> GAMVEATAQETDRPRFSFSIAAREGKARTGTIEMKRGVIRTPAFMPVGTAATVKALKPETVRATGADIILGNTYHLMLRPGAERIAKLGGLHSFMGWDRPILTDSGGYQVMSLSSLTKQSEEGVTFKSHLDGSRHMLSPERSIEIQHLLGSDIVMAFDECTPYPATPSRAASSMERSMRWAKRSRDAFDSRKEQAENAALFGIQQGSVFENLRQQSADALAEIGFDGYAVGGLAVGEGQDEMFRVLDFSVPMLPDDKPHYLMGVGKPDDIVGAVERGIDMFDCVLPTRSGRNGQAFTWDGPINIRNARFSE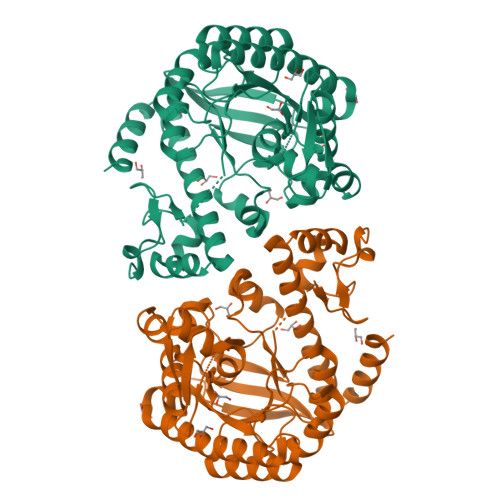DLKPLDSECHCAVCQKWSRAYIHDLIRAGEILGAMLMTEHNIAFYQQLMQKIRDSISEGRFSQFAQDFRARYFARNS>[4x]GAMGDVTK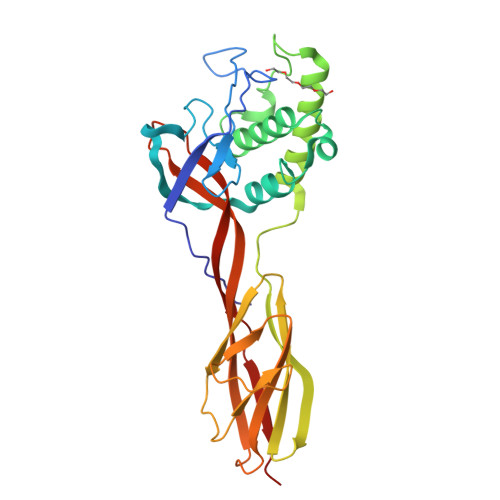PTSAKFIETGVKTDGYIRVNMPNHPNEWMISSQFKDSHGNIGYCMDSELPSPTGSGAGSLKYKGAGSDEFYRMFKGGFPSKTAKELGAGNDTEAWYATQLVSWVLAGNFKVSQIVWSHPNHTAAETARVKKAFEKIYDYAKNGKDTPNTEFSITASKTADEGKYHTFTYKTASNKTGNAKLTFTSAKPAGMKIYDADGKEITNNTVKLNSSFTIKVPVTTPSGTLSFKGTANVSTTNPFTFDGRGVYQDAVVMITTSETKDSKSLSAKWTRA>GSSKSWANHENKTVNKITVV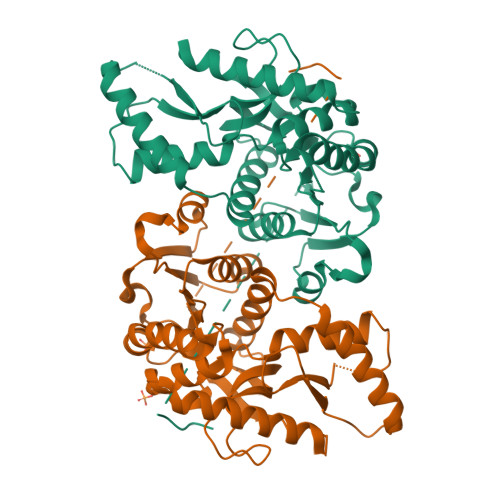GGGELGIACTLAISAKGIADRLVLLDLSEGTKGATMDLEIFNLPNVEISKDLSASAHSKVVIFTVNSLGSSQSYLDVVQSNVDMFRALVPALGHYSQHSVLLVASQPVEIMTYVTWKLSTFPANRVIGIGCNLDSQRLQYIITNVLKAQTSGKEVWVIGEQGEDKVLTWSGQEEVVSHTSQVQLSNRAMELLRVKGQRSWSVGLSVADMVDSIVNNKKKVHSVSALAKGYYDINSEVFLSLPCILGTNGVSEVIKTTLKEDTVTEKLQSSASSIHSLQQQLKL[2x]>DDDKMNLDFIKSKIAAVPDFPKPGIMFRDITPLLADPQGLRKTAEAMAQELKNKGIQPTIVAGTESRGFIFGVALAEVLGLGFVPVRKPGKLPRATYSVKYDLEYGSDSLEIHQDAFKVTDEVLVVDDLLATGGTAKATVDLIEKTQAKVAGLIFVMELDGLGGREV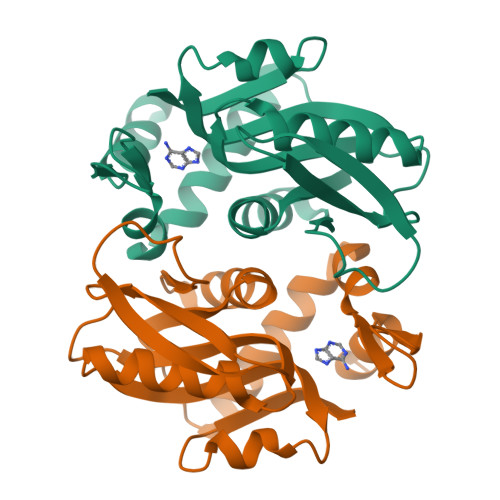LAGYNVSALIKF[4x]> GSMFTDWHEAAIGKTHNRMNFDCGDADLNQFLQRHARQNHEKGTTKTYVALDNSDVTRIHGFYSVSPASLIYAQVPGAISKGLGRYDVPVFRLGRLAVDKSMQGQGLGAQLLLSAGKRCIQAALQVGGVALLIDAKNKQVC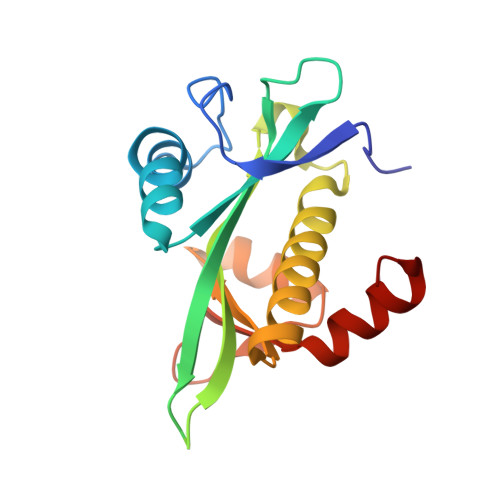DWFKGFGAVPLNDQPLSLLLSFKTLYAALSASGRL(phenylmethyl) N-[(2R)-2-[2-(4-bromanyl-3-oxidanyl-phenyl)-5-(methylcarbamoyl)benzimidazol-1-yl]-2-(3,4-dimethoxyphenyl)ethyl]carbamate | C33 H31 Br N4 O6 | 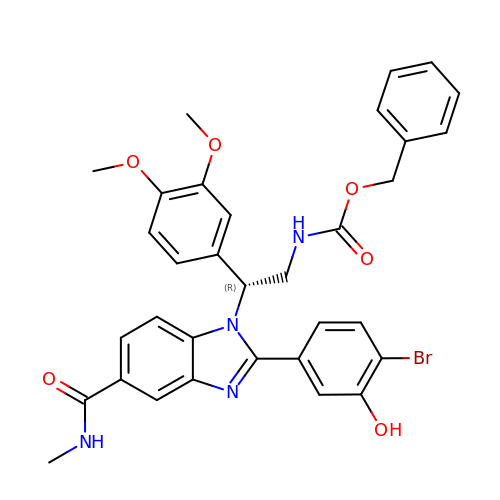JSBGVKZBZYECPF-MHZLTWQESA-N> MGHHHHHHENLYFQGSDVAIVKEGW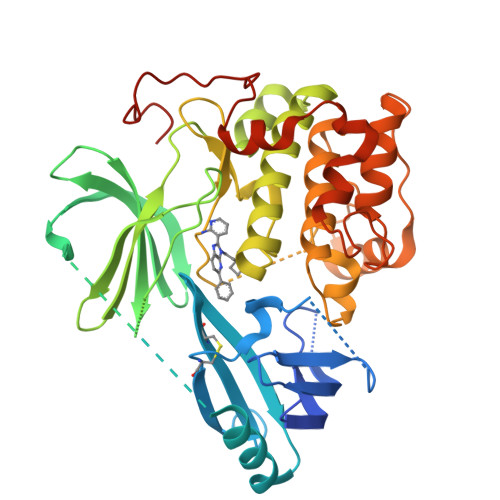LHKRGEYIKTWRPRYFLLKNDGTFIGYKERPQDVDQREAPLNNFSVAQCQLMKTERPRPNTFIIRCLQWTTVIERTFHVETPEEREEWTTAIQTVADGLKKQAAAEMDFRSGSPSDNSGAEEMEVSLAKPKHRVTMNEFEYLKLLGKGTFGKVILVKEKATGRYYAMKILKKEVIVAKDEVAHTLTENRVLQNSRHPFLTALKYSFQTHDRLCFVMEYANGGELFFHLSRERVFSEDRARFYGAEIVSALDYLHSEKNVVYRDLKLENLMLDKDGHIKITDFGLCKEGIKDGATMKTFCGTPEYLAPEVLEDNDYGRAVDWWGLGVVMYEMMCGRLPFYNQDHEKLFELILMEEIRFPRTLGPEAKSLLSGLLKKDPKQRLGGGSEDAKEIMQHRFFAGIVWQHVYEKKLSPPFKPQVTSETDTRYFDEEFTAQM To gain insight into the evolution and designability of ligand binding and specificity, we analyzed the homologous PBPs, PotF and PotD, which are Escherichia coli putrescine (PUT)-binding protein and spermidine (SPD)-binding protein, respectively. They constitute the first elements of two separate multicomponent uptake systems (PotFGHI and PotABCD) to transport the cationic polyamines PUT and SPD across the cellular membrane. Still, the protein-binding modes differ: PotF shows affinity for PUT and SPD, whereas PotD exclusively binds SPD. Prior to this work, we grafted the seven differences in amino acids from PotD binding pocket onto PotF; this resulted in PotF_SPD, which will be referred to as PotF/D throughout this work to keep naming for mutants more concise.

We introduced the S247D exchange into PotF/D and into our high-affinity constructs E39D–Y87S–F88Y and E39D–F88A/L. The combination of S247D with the other constructs led to an affinity improvement with which the nanomolar range was reached for the first time, while keeping the order of affinities in the different mutants the same compared with the prior analysis. Nonetheless, all constructs regained PUT affinity in the medium to low micromolar range. All structures but PotF/D–S247D adopt a fully closed wildtype conformation. PotF/D–E39D–Y87S–F88Y–S247D is the construct with the highest SPD affinity (840 nM). In this structure, Y88 is stacking with N65 and the salt bridge residue R91, stabilizing the latter and thereby adopting the fully closed conformation. Furthermore, the hydroxyl group of Y88 is coordinated by E66, whereas R91 is interacting with S87 in two alternate conformations. Taken together, the interplay of the mentioned residues forms a tight pocket surrounding Y88, thereby stabilizing the distal region and supporting the completely closed conformation. In all constructs that carry S247D, SPD adopts a “relaxed” conformation and does not show unexpected bending of its backbone to fit a specific position as it does when being bound by PotF wildtype or PotF/D. On the other hand, we designed a PotF/D construct that completely switched its ligand preference compared with the wildtype by exhibiting nanomolar affinity for SPD (840 nM) and medium micromolar affinity for PUT (88 μM).

>[2x]AEQKTLHIYNWTDYIAPDTVANFEKETGIKVVYDVFDSNEVLEGKLMAGSTGFDLVVPSASYLERQLTAGVFQPLDKSKLPEWKNLDPELLKLVAKHDPDNKFAMPYMWATTGIGYNVDKVKAVLGENAPVDSWDLILKPENLEKLKSCGVSFLDDPEEVFATVLNYLGKDPNSTKADDYTGPATDLLLKLRPNIRYFHSSQYINDLANGDICVAIGWAGDVWQASNRAKEAKNGVNVSFSIPKEGAMAWFDVFAMPADAKNKDEAYQFLNYLLRPDVVAHISDHVFYANANKAATPLVSAEVRENPGIYPPADVRAKLFTQKVQDPKIDRVRTRAWTKVKSGKLEHHHHHH> MLLEEVRAGDRLSGAAARGDVQEVRRL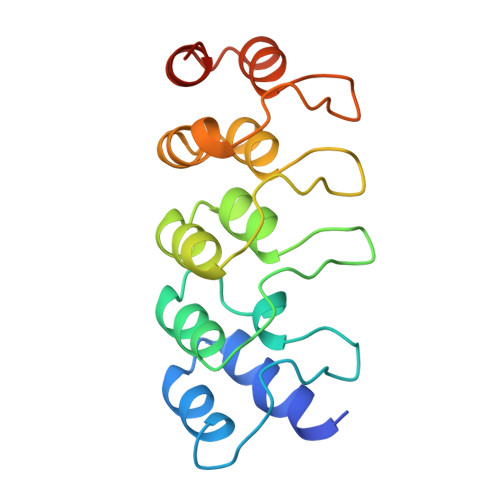LHRELVHPDALNRFGKTALQVMMFGSTAIALELLKQGASPNVQDTSGTSPVHDAARTGFLDTLKVLVEHGADVNVPDGTGALPIHLAVQEGHTAVVSFLAAESDLHRRDARGLTPLELALQRGAQDLVDILQGHMVAPL>LLGDFFRKSKEKIGKEFKRIVQRIK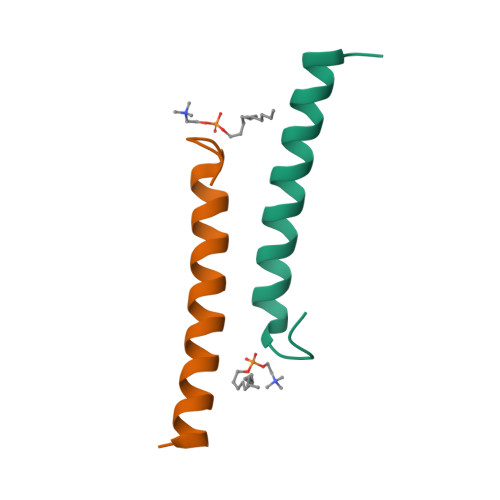DFLRNLVPRTES[2x]>[4x]TMSLQVDLLNNTFANPFMNAAGVMCSTTEDLVAMTESASGSLVSKSCTPALREGNPTPRYRALPLGSINSMGLPNNGFDFYLAYAAEQHDYGRKPLFLSMSGLSVRENVEMCKRLAAVATEKGVILELNLSCPNVPGKPQVAYDFDAMRQCLTAVSEVYPHSFGVKMPPYFDFAHFDAAAEILNEFPQVQFITCIN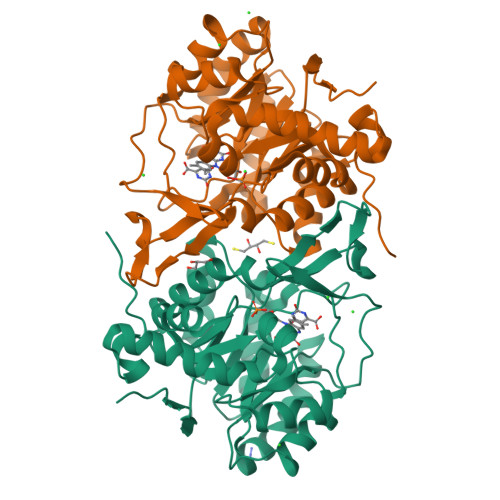SIGNGLVIDAETESVVIKPKQGFGGLGGRYVLPTALANVNAFYRRCPGKLIFGCGGVYTGEDAFLHVLAGASMVQVGTALHEEGPAIFERLTAELLDVMAKKGYQTLDEFRGKVRTLD> MDSDEHLYKLKTFLENLRRHLDRLDKHIKQLRDILSENP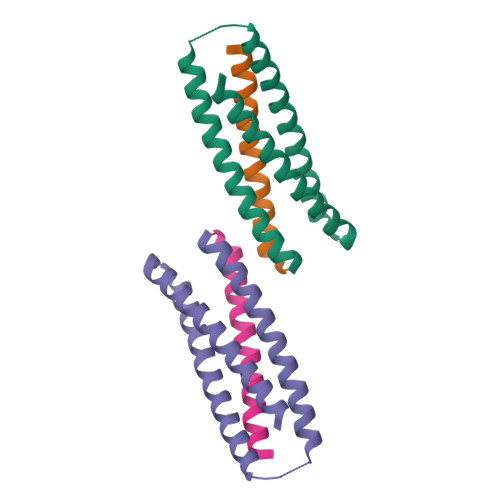EDERVKDAIDLSERSVRIVKTVIKIFEDSVRKKEKRPIDKRDDKELDKLLDTLEKILQTATKIIDDANKLLEYLRR;> HGDPKVVETYVELLKRHEKAVKELLEIAKTHAKKVE4-(3-amino-1H-indazol-5-yl)-N-tert-butylbenzenesulfonamide 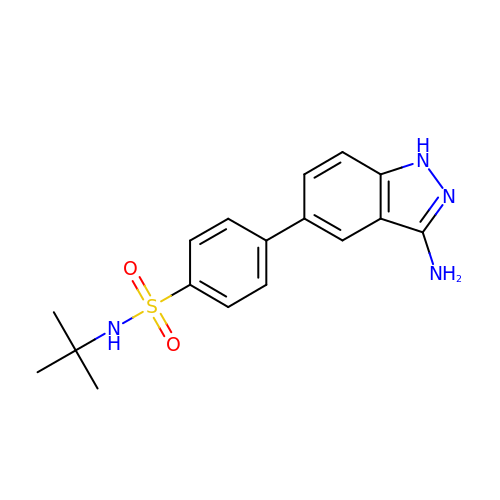| C17 H20 N4 O2 S | KFJCXIOVAGJCKB-UHFFFAOYSA-N>RKRNRIPLSCTICRKRKVKCDKLRPHCQQCTKTGVAHLCHYMEQTWAEEAEKELLKDNELKKLRERVKS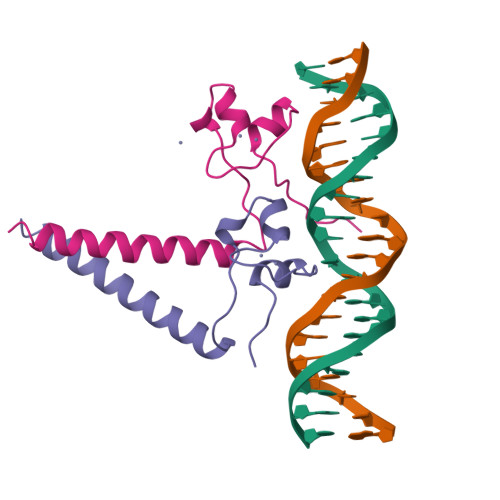LEKTLSKVHSSP[4x]E. coli cytolysin A (ClyA), also known as hemolysin (HlyE) or silent hemolysin A (SheA), belongs to the α-PFT class. ClyA is a 34 kDa soluble monomer, containing mainly α-helices with only one β-tongue that transforms into α-helical elements in the pore complexes. Each protomer in the ClyA pore complexes is composed of five α-helices, namely αA1, αB, αC, αF, and αG. Here we report the cryo-EM structures of ClyA pore complexes in the presence of n-Dodecyl-β-D-Maltoside (DDM) as dodecamer, tridecamer, and tetradecamer at the resolution of 2.8 Å, 3.2 Å and 4.3 Å, respectively.

Soluble ClyA monomer was previously found to assemble into a 13-meric pore complex in the presence of DDM, but a dodecamer was observed in the crystal structure. Two top view images (or bottom view, as they cannot be differentiated) clearly indicated the presence of both dodecamer and tridecamer. Based on the particle numbers of total particles and those used in final 3D reconstructions, the majority of the complexes were 12-meric, representing approximately 80% of all particles, while only 11% were 13-meric. These observations confirm the existence of 13-metric ClyA pore complexes, albeit at a low concentration in this preparation. Final 3D reconstruction resulted in EM density maps of the dodecamer, the tridecamer and the tetradecamer at the resolution of 2.8 Å, 3.2 Å and 4.3 Å, respectively. The near-atomic resolution maps of the dodecamer and the tridecamer allowed reasonable model building with accurate side chain assignments. The inner diameters near the extracellular edge of the pore are 70, 72 and 77 Å for the dodecamer, the tridecamer, and the tetradecamer, respectively. Comparison between Prot_12 and a protomer from the tridecamer (Prot_13) or the tetradecamer (Prot_14) shows that the overall fold of the protomer does not change when forming various oligomers, indicating a rigid body protomer assembly mechanism for the ClyA pore complexes. The interaction paradigm remains highly conserved in the tridecamer, suggesting a single protomer-protomer interaction mode in the ClyA pore complexes. The protomer-protomer interaction paradigm in the dodecamer applies also to the tridecamer, and probably the tetradecamer.

>[13x]MGSSHHHHHHSQDLDEVDAGSMTEIVADKTVEVVKNAIETADGALDLYNKYLDQVIPWQTFDETIKELSRFKQEYSQAASVLVGDIKTLLMDSQDKYFEATQTVYEWCGVATQLLAAYILLFDEYNEKKASAQKDILIKVLDDGITKLNEAQKSLLVSSQSFNNASGKLLALDSQLTNDFSEKSSYFQSQVDKIRKEAYAGAAAGVVAGPFGLIISYSIAAGVVEGKLIPELKNKLKSVQNFFTTLSNTVKQANKDIDAAKLKLTTEIVAIGEIKTETETTRFYVDYDDLMLSLLKEAAKKMINTCNEYQKRHGKKTLFEVPEV> GEYASVTDVYNYYKYGELLRGGICHSVQLTAAISNGCIKNGKHNIFIIGDSYAAALFNGLSHYIDNKGSDYIISQMTDGNAPPLFVDGKDDLQRSVITLNNNRINEIKRVQPEVVLLTWSVRGTNGVHDKKLAIDALSLTIKKIKEASPDSRIIFIGPVPEWNANLVKIISNYLSEFKKTPPLYMTYGLNSEISEWDSYFSNNVPKMGIEYISAYKALCNESGCLTRVGNGPDFITAVDWGHLTKPGSDFLFNKIGNKIIK

O-antigen acetylation by AT3 domain-containing acetyltransferases of Salmonella spp. can generate a specific immune response upon infection and can influence bacteriophage interactions. This study integrates in situ and in vitro functional analyses of two of these proteins, OafA and OafB (formerly F2GtrC), which display an “AT3-SGNH fused” domain architecture, where an integral membrane AT3 domain is fused to an extracytoplasmic SGNH domain. Multiple Salmonella serovars have a rhamnose moiety in the O-antigen that can be acetylated at the 2- and 3-hydroxyl groups by F2GtrC proteins. In AT3-SGNH proteins, the AT3 domain passes an acetyl group from an unidentified donor in the cytoplasm to the periplasmic face of the inner membrane. This acetyl group is then transferred to the SGNH domain, which catalyzes specific carbohydrate O-acetylation.

We expressed and purified residues 366 to 609 from OafA (OafA-STMC-long) and residues 377 to 640 from S. Paratyphi OafB (OafB-SPAC-long), which have 31% sequence identity. No diffracting crystals of OafA-STMC-long were obtained; however, crystals diffracting to a 1.1-Å resolution were obtained for OafB-SPAC-long, with a single molecule in the asymmetric unit. The structure could not be solved by molecular replacement using a number of known SGNH structures but was solved using Fragon with a 14-residue ideal polyalanine α-helix as the search model and refined to an Rwork/Rfree of 13.6/14.9%. The core structure of OafB-SPAC-long resembles an SGNH domain with an α/β/α hydrolase fold consisting of five central β-strands surrounded by six α-helices. Two disulfide bonds are seen in the structure and were verified using mass spectrometry. Second, and most significantly, the region that connects the end of TM11 and the start of the sequence of other known SGNH domains (residues 377 to 421) is clearly structured and forms a long extension of the SGNH domain that we now term the SGNH extension (SGNHext). The SGNHext interacts extensively with the SGNH domain covering 1,500 Å2 of the SGNH domain, including interactions with helix α8; 38 amino acids of the SGNH domain interact with 32 (of 48) residues in the extension. The structure of OafB-SPAC-long shows OafBN459 to be within hydrogen-bonding distance of a cocrystallized sulfate ion, suggesting that OafBN459 could interact with bound substrate and participate in oxyanion hole formation. OafB-SPAC-long contains a GTNG motif (OafBG502-G505) close to sequence block III, but the side chains of these residues are oriented away from the catalytic triad.>[2x]MTTNVALVGLARDLAARAETGKPIRIGLIGAGEMGTDIVTQVARMQGIEVGALSARRLPNTFKAIRTAYGDEENAREATTESAMTRAIEAGKIAVTD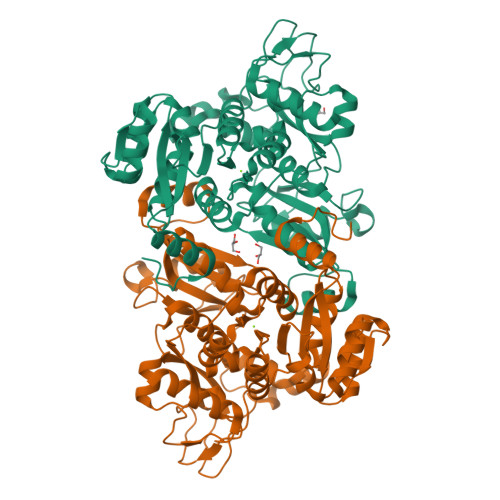DNDLILSNPLIDVIIDATGIPEVGAETGIAAIRNGKHLVMMNVEADVTIGPYLKAQADKQGVIYSLGAGDEPSSCMELIEFVSALGYEVVSAGKGKNNPLNFDATPDDYRQEADRRNMNVRLLVEFIDGSKTMVEMAAIANATGLVPDIAGMHGPRASIDQLSHTLIPQAEGGVLSKSGVVDYSIGKGVSPGVFVVAKMDHPRLNERLEDLKIGKGPYFTFHRPYHLTSLEVPLTVARVVLHGKTDMVPLPKPVAEVCAVAKKDMQPGEHLDAIGQYCYRSWIMTVPEARAAKAIPCGLLQNGTVIAPIKKGELITYANAAPQPGSRIAELRALQDAMLGQLEHHHHHH> SYRPYA;> MHHHHHHMQIGWRREGIKYRRNELFLDVLESVNLLMSPQGQVLSAHVSGRVVMKSYLSGMPECKFGMNDKIVIEKQGKGTADETSKSGKQSIAIDDCTFHQCVRLSKFDSE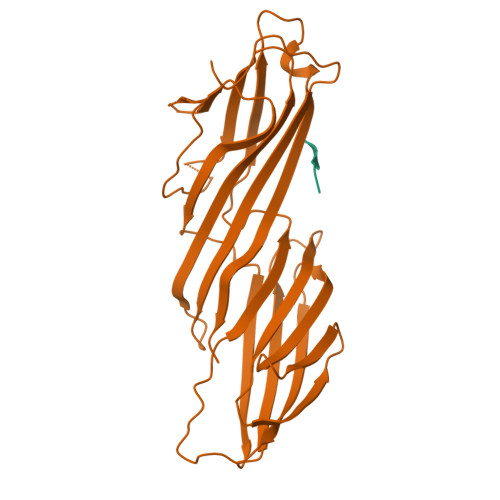RSISFIPPDGEFELMRYRTTKDIILPFRVIPLVREVGRTKLEVKVVIKSNFKPSLLAQKIEVRIPTPLNTSGVQVICMKGKAKYKASENAIVWKIKRMAGMKESQISAEIELLPTNDKKKWARPPISMNFEVPFAPSGLKVRYLKVFEPKLNYSDHDVIKWVRYIGRSGIYETRC>MLVSVYLALLVACVGQAHSQANLMRLKSDLFNRSPMYPGPTKDDPLTVTLGFFLQDIVKVDSSTNEVDLVYYERQRWKLNSLMWDPNEYGNITDFRTSAADIWTPDITAASSTRPVQVLSPQIAVVTHDGSVMFSPAQRLSFMCDPTGVDSEEGVTCAVKFESWVYSGFEIDLKTDTDQVDLSSYYASSKYEILSATQTRQVQHYSCCPEPYIDVNLVVKFRERRAGNGFFRNLFDENLYFQGHHHHHH[15x]

Protein-engineering methods have been exploited to produce a surrogate system for the extracellular neurotransmitter-binding site of a heteromeric human ligand-gated ion channel, the glycine receptor. Acetylcholine-binding protein is a highly conserved ortholog of the pLGIC extracellular ligand-binding domain (ECD) with properties similar to nAChR. Mutations affecting key residues in the orthosteric agonist site at the α1(−)/β(+) interface affect the potency of both activation by glycine and inhibition by strychnine. We therefore set out to generate a high-fidelity surrogate of this α1(−)/β(+) orthosteric binding site using the 2α1:3β stoich­iometry [Fig. 1(a)] by exploiting protein-engineering methods and the thermal stability of acetylcholine-binding protein from Aplysia californica (AcAChBP). Ultimately, the highly stable AcAChBP framework has allowed us to introduce nine amino-acid substitutions that have resulted in a stable surrogate for a heteromeric neurotransmitter site that binds glycine.

Variant II therefore reverted back to Trp164, but with the inclusion of a G162E substitution. The residues now changed (Thr53, Gln74, Tyr110, Ile135 and Gly162) correspond to Phe72, Arg93, Ala146, Ser157 and Glu202 in the human GlyR-α1(−)/β(+) orthosteric site [Figs. 1(b) and 2]. Crystal structures of variant II with HEPES, tropisetron and strychnine revealed that the G162E substitution was accommodated with the structure essentially unperturbed compared with variant I, although now incorporating two charged residues (Arg74 and Glu162) to polarize the binding site such that the principal side is negatively charged and the complementary side is positive. The incorporation of the inter-strand hydrogen bond between Trp164 and Ile135 is likely to support this recovery of thermal stability.>[4x]MDIGINSDPPPRDWQLEKVVELSRAGIRPPTAGNREAIEAATGRPWTEWTTHDGELTGHGYAAVVNKGREEGQHYRQLGLLQAGCPTAESIYVRASPLQRTRATAQALVDGAFPGCGVAIHYANGDADPLFQTDKFAATQTDPARQLAAVKEKAGDLAQRRQALAPTIQLLKQAVCQADKPCPIFDTPWRVEQSKSGKTTISGLSVMA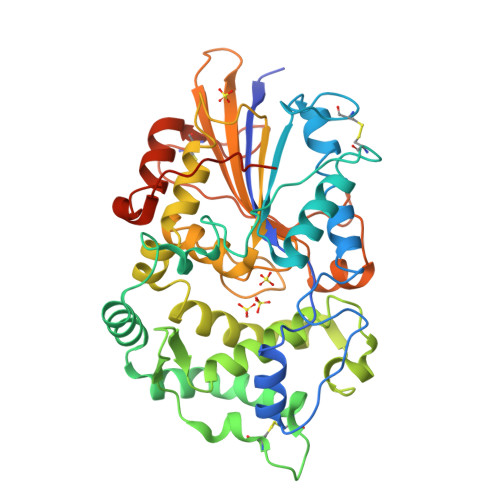NMVETLRLGWSENLPLSQLAWGKIAQASQITALLPLLTENYDLSNDVLYTAQKRGSVLLNAMLDGVKPEASPNVRWLLLVAHDTNIAMVRTLMNFSWQLPGYSRGNIPPGSSLVLERWRDAKSGERYLRVYFQAQGLDDLRRLQTPDAQHPMLRQEWRQPGCRQTDVGTLCPFQAAITALGQRIDRPSAPAVAMVLPKLAAALEHHHHHH>GSDKIHHHHHHMLTMKDIIRDGHPTLRQKAAELELPLTKEEKETLIAMREFLVNSQDEEIAKRYGLRSGVGLAAPQINISKRMIAVLIPDDGSGKSYDYMLVNPKIVSHSVQEAYLPTGEGCLSVDDNVAGLVHRHNRITIKAKDIEGNDIQLRLKGYPAIVFQHEIDHLNGVMFYDHIDKN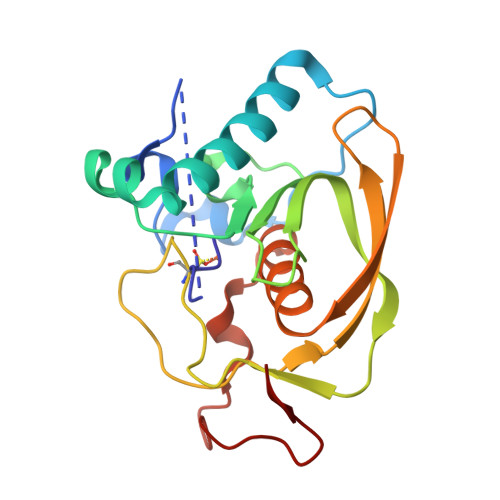HPLQPHTDAVEV[2x]>[2x]HMSIITDVYAREVLDSRGNPTLEVEVYTESGAFGRGMVPSGASTGEHEAVELRDGDKSRYLGLGTQKAVDNVNNIIAEAIIGYDVRDQQAIDRAMIALDGTPNKGKLGANAILGVSIAVARAAADYLEVPLYTYLGGFNTKVLPTPMMNIINGGSHSDAPIAFQEFMIMPVGAPTFKEGLRWGAEVFHALKKILKERGLVTAVGDE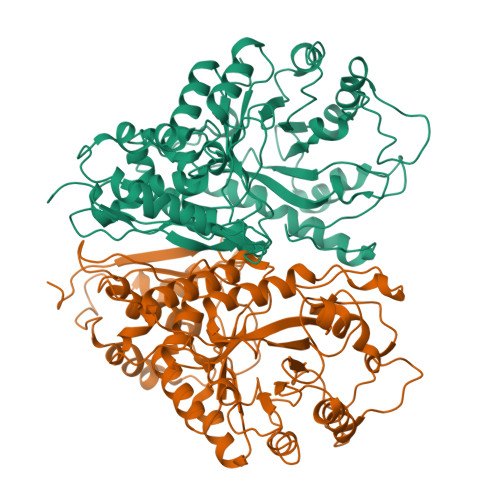GGFAPKFEGTEDGVETILKAIEAAGYEAGENGIMIGFDCASSEFYDKERKVYDYTKFEGEGAAVRTSAEQVDYLEELVNKYPIITIEDGMDENDWDGWKVLTERLGKRVQLVGDDFFVTNTEYLARGIKENAANSILIKVNQIGTLTETFEAIEMAKEAGYTAVVSHRSGETEDSTIADIAVATNAGQIKTGSLSRTDRIAKYNQLLRIEDQLGEVAQYKGIKSFYNLKK>[2x]SNAMLENIRIVLIETSHSGNIGSAARAMKTMGLTQLCLVSPKSVDEQSYALSAGAENIVKNARVVDSFDE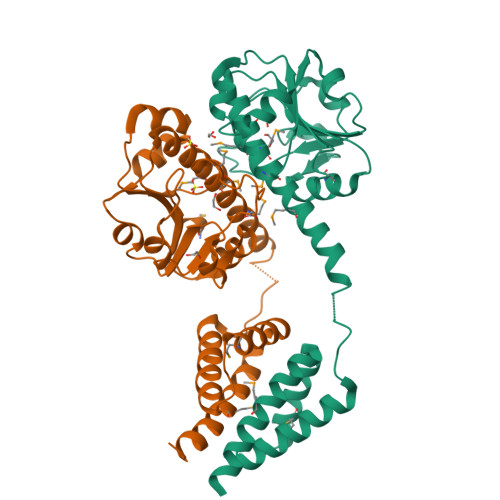AVDDCSLVIGTSARLRHLQNTLIEPRECAEKVVAYKGKIAIVFGRERIGLTNEELLKCHYHLNIPANPDYSSLNLAMAVQLVSYELRMAFLVQNNKKNSLSLIEKNYPTTDQLAYFFDYTERIYQSLGFIQNQGVMRKLKRLYYRAKLEKNELNILNGMLSAVEKRIDLTKEDN>MGQDHIRYDILAQDALRGVIRKVLGEVAATGRLPGDHHFFITFLTGAPGVRISQHLKSKYAEQ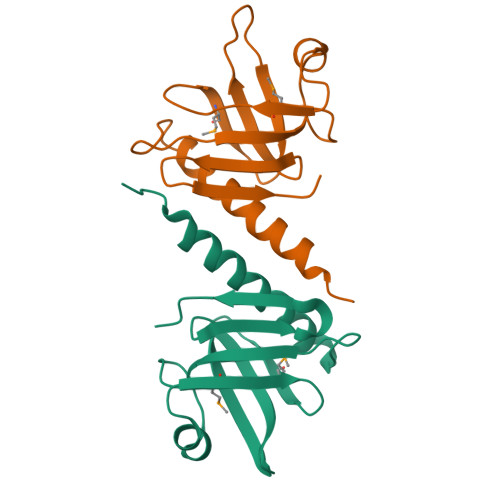MTIVIQHQFWDMKVTETGFEIGLSFSDTPEKLVIPYNAIRGFYDPSVNFELEFDVPLAKEEEMEEAEITAYPVSHEAKPASETPKSGEEKKEGSVVSLDAFRKKQLEHHHHHH[2x]>[3x]EEEERAFLVAREELASALRRDSGQAFSLEQLRPLLASSLPLAARYLQLDAARLVRCNAHGEPRNYLNTLSTALNILEKYGRNLLSPQRPRYWRGVKFNNPVFRSTVDAVQGGRDVLRLYGY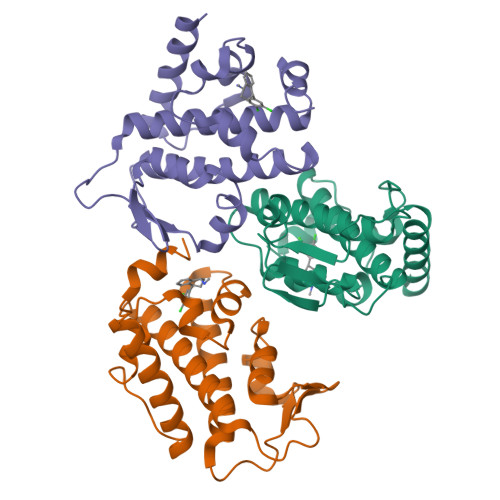TEEQPDGLSFPEGQEEPDEHQVATVTLEVLLLRTELSLLLQNTHPRQQALEQLLE> SNAMHMLRIAKEALTFDDVLLVPAHSTVLPNTADLRTRLTKNIALNIPMVSASMDTVTEARLAIALAQEGGIGFIHKNMSIEQQAAQVHQVKISGGLRVGAAVGAAPGNEERVKALVEAGVDVLLIDSSHGHSE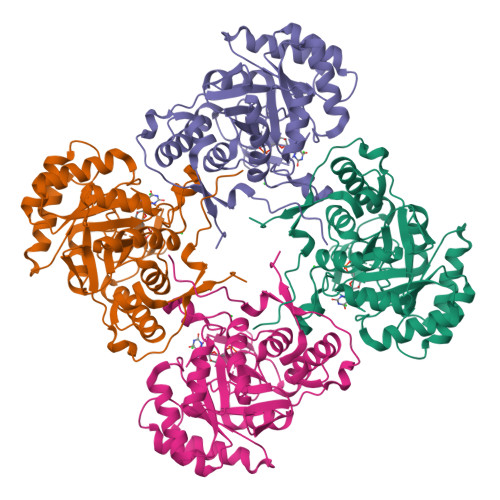GVLQRIRETRAAYPHLEIIGGNVATAEGARALIEAGVSAVKVGIGPGSICTTRIVTGVGVPQITAIADAAGVANEYGIPVIADGGIRFSGDISKAIAAGASCVMVGSMFAGTEEAPGEVILYQGRSYKAYRGMGSLGAMSKGSSDRYFQTDNAADKLVPEGIEGRIAYKGHLKEIIHQQMGGLRSCMGLTGSATVEDLRTKAQFVRISGAGMKESHVHDVQITKEAPNYRLG> GHMSYDRVKDFDLPELAVHLQPHGAVMIDRKSMFYFRLSGRGAQLAFLLSKNKNLHKTARIWEIMKKEEMSADQLKEELSAHPFTEAWTEGLLDQPLHVSGSLDSYLPISCTLQLTNACNLSCSFCYASSGKPYPEELSSEQWILVMQKLAAHGVADITLTGGEAKLIKGFKELVVVASSLFTNVNVFSNGLNWRDEEVELLSHLGNVSVQISIDGMDNTHDQLRGRKGGFKESMNTIKKLSEANIPVIVAMTINESNADEVSDVVEQCANAGAFIFRAGKTLSVGRATEGFKALDIDFEEMVQIQLREARHKWGDRLNIIDWEHEESSFTTDF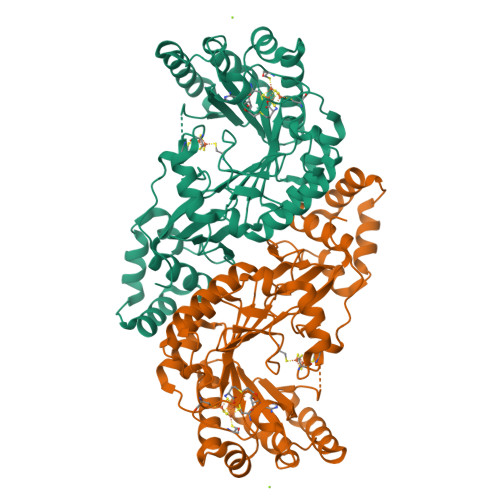CTPGYLAWYIRADGYVTPCQLEDLPLGHILEDSMADIGSPARLLQLKCEAKNCKCIGKIELSEPDLPFQKEVKAGIQE>GCGAATTCG[2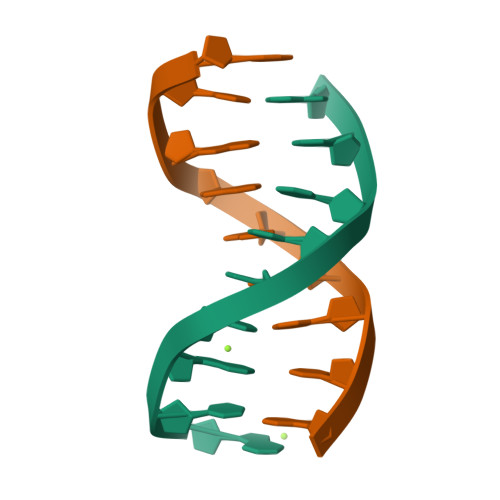x]> MSEVITVKQTNMENIYECEFNDGSFRLCTRNLVPNFNVYGERLIKYEGVEYREWNAFRSKLAGAILKGLKTNPIRKGTKVLYLGAASGTTISHVSDIIELNGKAYGVEFSPRVVRELLLVAQRRPNIFPLLADARFPQSYKSVVENVDVLYVDIAQPDQTDIAIYNAKFFLKVNGDMLLVIKARSID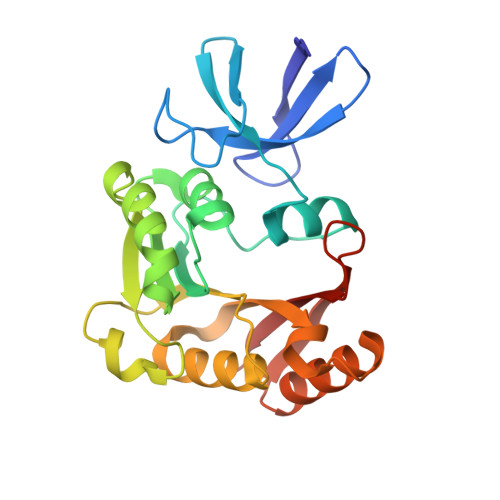VTKDPKEIYKTEVEKLENSNFETIQIINLDPYDKDHAIVLSKYKG>MKQYLELMQKVLDEGTQKNDRT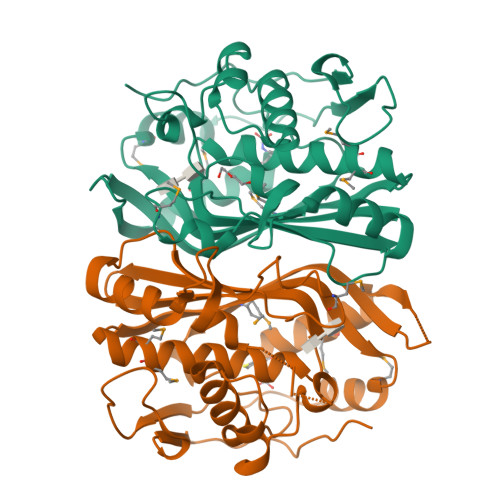GTGTLSIFGHQMRFNLQDGFPLVTTKRCHLRSIIHLLLWFLQGDTNIAYLHENNVTILDEWADENGDLGPVHGKQWRAWPTPDGRHIDQITTVLNQLKNDPDSRRIIVSAWNVGELDKMANAPSHAFFQFYVADGKLSCQLYARSEDVFLSLPFAIASGALLVHMMAQQCDLEVGDFVMTGGDTHLYSNHMDQTHLQLSREPRPLPKLIIKRKPESIFDYRFEDFEIEGYDPHPGIKAPVAILEHHHHHH[2x]> MTDGLNQLYNLVAQDYALTDTIEALSRMLHRGTIPLDTFVKQGRE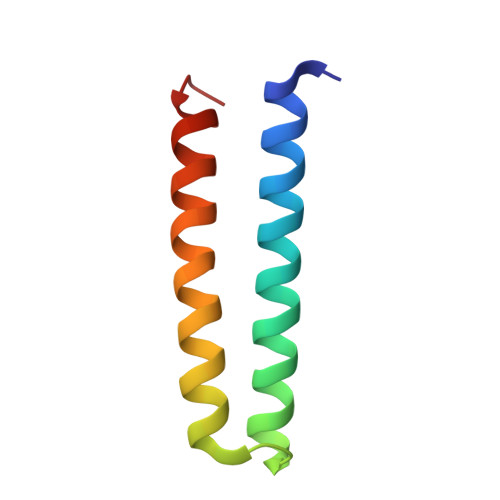LARQQFLVRWHIQRITSPLS XIAP (X-linked inhibitor of apoptosis) directly inhibits the upstream caspase-9 and the downstream caspase-3 and caspase-7, and therefore controls critical apoptotic checkpoints. The XIAP protein consists of several domains, including three zinc-containing BIR (baculovirus IAP repeat) domains (BIR1, BIR2 and BIR3) and a C-terminal RING domain. The linker region blocks the active sites of these caspases, while the N-terminal regions of the partially processed caspase-3 and caspase-7 bind the BIR2 domain in a peptide-binding groove that accommodates the four N-­terminal residues. As has been reported previously for other BIR domains, the overall architecture of the BIR2 domain is a three-stranded antiparallel β-sheet surrounded by five α-helices, with a structurally important zinc residue coordinated by Cys200, Cys203, His220 and Cys227.

Therefore, the structures of XIAP BIR2 with five different peptides soaked in and bound to the Smac binding groove were also solved: ATAA, AVPI, SVPI, AIAV and AMRV. Replacing the N-terminal alanine with a serine causes a loss of activity for both BIR2 and BIR3, although this is a conservative change. The crystal structures of BIRC1 and BIRC3 and XIAP BIR2–caspase-3 all have an N-terminal serine at the P1 position; the Oγ H atom is within hydrogen-bonding distance of the glutamine at the edge of the pocket. Even with a serine at P1, the P1–P3 residues bind nearly identically. However, the P4 isoleucine is much larger than alanine, and even though Gln197 rotates away from the pocket (in fact, Gln197 has two alternate conformations in this structure), the larger pocket created by this movement is still not large enough to accommodate the isoleucine side chain without a shift in the backbone. The position of SVPI in BIR2 aligns well with most published BIR domain–AVPI structures. The additional hydroxyl introduced by the serine substitution results in only a small shift in the side chains of His223 and Leu207 to allow the extra atom. Next, AIAV binds identically to SVPI, but with an intermediate position observed for Gln197, which does not have to move as much to accommodate the valine as it does for the isoleucine. This series of structures highlights the flexibility of the protein and the value of having multiple structures for comparison.

>GTIYPRNPAMYSEEARLKSFQNWPDYAHLTPRELASAGLYYTGIGDQVQCFACGGKLKNWEPGDRAWSEHRRHFPNCFFVLGRNLN[2x];> SVPI>MLEARLEQASLLKRVVDAIKDLVQDCNFDCNDSGIALQAMDNSHVALVSMLLKAEGFSAYRCDRNIALGINLVSLTKVLRAAQNEDILTLKADDSPDAVNLMFESAETDRISEYDIKLMDIDQEHLAIPETEYAATVE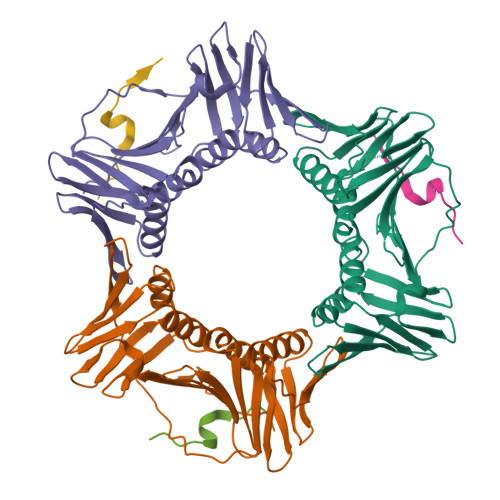MPSAEFQRICRDLNALSESVVIEATKEGVKFSCQGDIGSGSVTIRQHTSVDKPEQNVSIALSEPVALTFSLKYLVNFCKATSLSSKVTLCLSQEVPLLVEYGLGSGHLRFYLAPKIGD[3x];>KRRQTSMTDFYHSKR[3x]> MNDHFVKRPKLELSDPSEPLTQKDVIAFQKEALFRC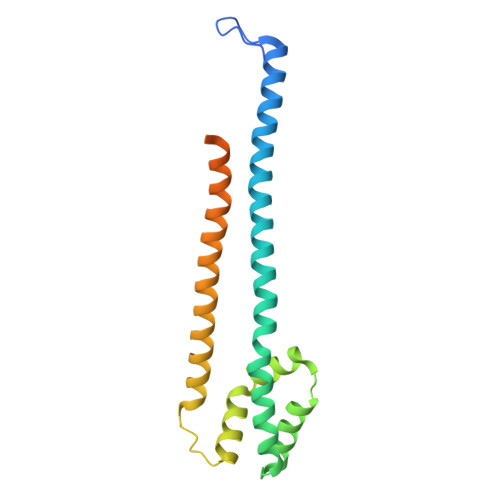LNKWRVKANQLVEENEVLAAGLSKTTESVSGCCSSIVVLARSVVEDCSDEQDKRFLQQLINTEDEHTLTQIISNNSARICELILKTSGSNISDNIGRLQELESLTLTLQKLLKSSENKLKKATEYYENIIAQYDRQDSESVSRVFNTADDDSNVKKEKQSSTGASSVNDE>ASAGVAVTNLNLKPGHCVEIKGSIPPDCKGFAVNLGEDASNFLLHFNARFDLHGDVNKIVCNSKEADAWGSEQREEVFPFQQGAEVMVCFEYQTQKIIIKFSSGDQFSFPVRKVLPSIPFLSLEGLAFKSITTE[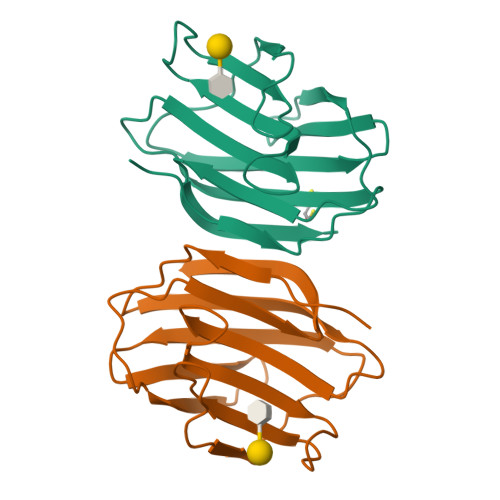2x]> KKSAKDALLLWCQMKTAGYPNVNIHNFTTSWRDGMAFNALIHKHRPDLIDFDKLKKSNA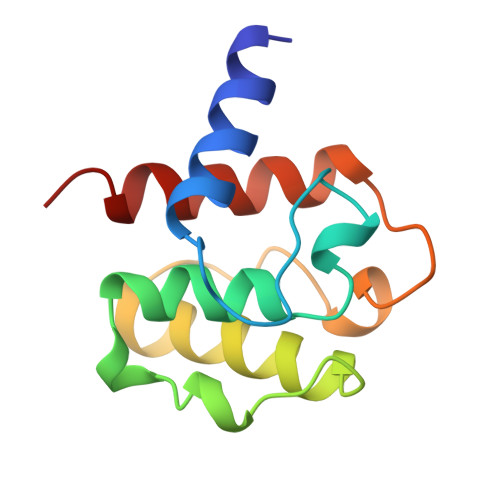HYNLQNAFNLAEQHLGLTKLLDPEDISVDHPDEKSIITYVVTYYHYFSKM> GPHMTVFHDKENFNVKHPLSCRWTLWFTK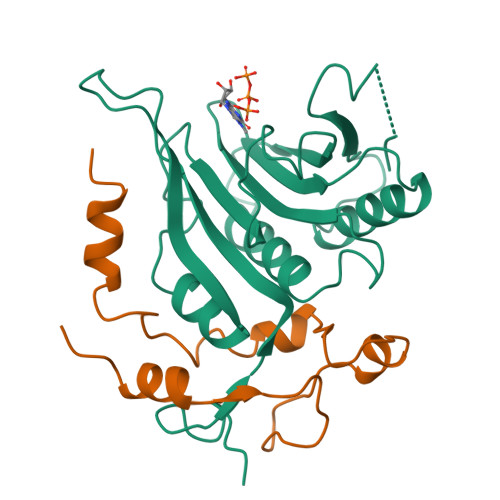PASGKGDNWNDLLKKVITFESVEEFWGIYNNIAPVSELAVKSDYHLFKEGVRPEWEDPQNKHGGKWAYQFKDKRSVNIDELWLHTMLAAIGETLEDEEDGEVMGVVVNVRKGFYRIGVWTRTTEKSKEILMNIGRRLKEVLKLPPNEMVEFSGHTEAAQAGSTRAKARMVV;> GPHMQPSAALQSLRSARFLPGIVQDIYPPGIKSPNPALNEAVQKKGRIFKYDVQFLLQFQNVFTEKPSPDFDQQVKALIGD>MSTAGDGERGTVGQEDSAAAMPFRFSPEPTLEDIRRLHAEFAAERDWEQFHQPRNLLLALVGEVGELAELFQWKSDTEPGPQAWPPKERAALQEELSDVLIYLVALAARC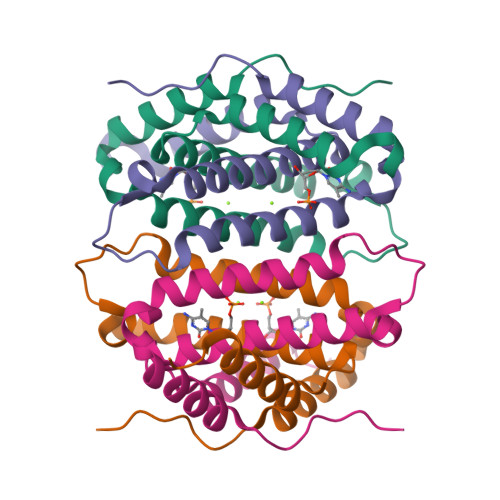HVDLPQAVISKMDTNRQRYPVHLSRGSACKYTDLPRGTISENQAVGAGDPASELRDQAST[2x]>[4x]MMSGEHTLKAVRGSFIDVTRTIDNPEEIASALRFIEDGLLLIKQGKVEWFGEWENGKHQIPDTIRVRDYRGKLIVPGFVDTHIHYPQSEMVGAYGEQLLEWLNKHTFPTERRYEDLEYAREMSAFFIKQ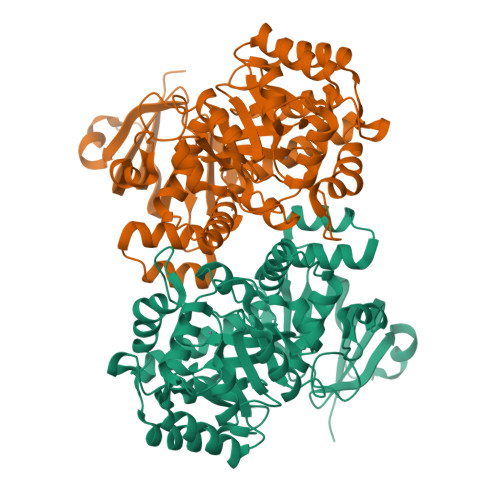LLRNGTTTALVFGTVHPQSVDALFEAASHINMRMIAGKVMMDRNAPDYLLDTAESSYHQSKELIERWHKNGRLLYAITPRFAPTSSPEQMAMAQRLKEEYPDTWVHTHLCENKDEIAWVKSLYPDHDGYLDVYHQYGLTGKNCVFAHCVHLEEKEWDRLSETKSSIAFCPTSNLYLGSGLFNLKKAWQKKVKVGMGTDIGAGTTFNMLQTLNEAYKVLQLQGYRLSAYEAFYLATLGGAKSLGLDDLIGNFLPGKEADFVVMEPTATPLQQLRYDNSVSLVDKLFVMMTLGDDRSIYRTYVDGRLVYERN> MGAKYKKEFAAYTAALAEAESK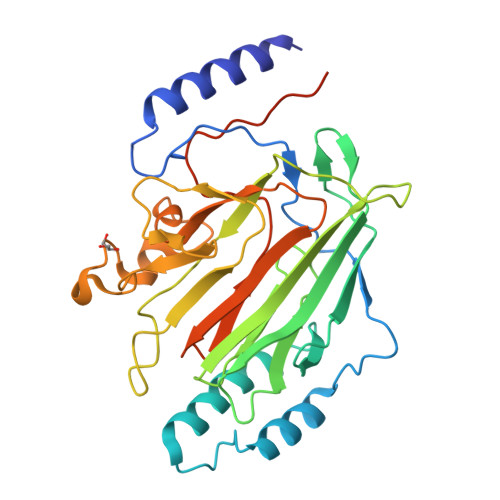KKQDGYLSEPRSQSLNFKSEPNAIRTIDSSVHQYGQQELDALVKSWGISPTNPDRKKSTAYSYFNAINSNNTYAKLVLEKDKPVDVTYTGLKNSSFNGKKISKVVYTYTLKETGFNDGTKMTMFASSDPTVTAWYNDYFTSTNINVKVKFYDEEGQLMNLTGGLVNFSSLNRGNGSGAIDKDAIESVRNFNGRYIPISGSSIKIHENNSAYADSSNAEKSLGARWNTSEWDTTSSPNNWYGAIVGEITQSEISFNMASSKSGNIWFAFNSNINAIGVPTKPVAPTENLYFQGAAALEHHHHHH>MESKRLDNAALAAGISPNYINAHGKPQSISAETKRRLLDAMHQRTATKVAVTPVPNVMVYTSGKKMPMVVEGSGEYSWLLTTEEGTQYKGHVTGGKAFNLPTKLPEGYHTLTLTQDDQRAHCRVIVAPKRCYEPQALLNKQKLWGACVQLYTLRSEKNWGIGDFGDLKAMLVDVAKRGGSFIGLNPIHALYPANPESASPYSPSSRRWLNVIYIDVNAVEDFHLSEEAQAWWQLPTTQQTLQQARDADWVDYSTVTALKMTALRMAWKGFAQRDDEQMAAFRQFVAEQGDSLFWQAAFDALHAQQVKEDEMRWGWPAWPEMYQNVDSPEVRQFCEEHRDDVDFYLWLQWLAYSQFAACWEISQGYEMPIGLYRDLAVGVAEGGAETWCDRELYCLKASVGAPPDILGPLGQNWGLPPMDPHIITARAYEPFIELLRANMQNCGALRIDHVMSMLRLWWIPYGETADQGAYVHYPVDDLLSILALESKRHRCMVIGEDLGTVPVEIVGKLRSSGVYSYKVLYFENDHEKTFRAPKAYPEQSMAVAATHDLPTLRGYWECGDLTLGKTLGLYPDEVVLRGLYQDRELAKQGLLD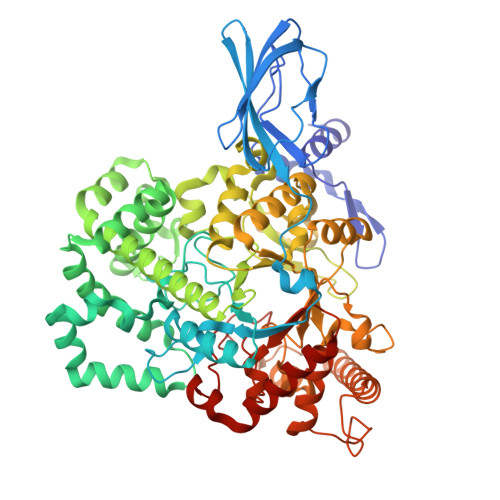ALHKYGCLPKRAGHKASLMSMTPTLNRGLQRYIADSNSALLGLQPEDWLDMAEPVNIPGTSYQYKNWRRKLSATLESMFADDGVNKLLKDLDRRRRSAHHHHHH[2x]> MGIVEEAHNVKVLGTGSRFIVLAHGFGTDQSVWKHLVPHLLEEFRVILYDNMGAGTTNPDYFDFERYSTLEGYAYDLLAILQELRVDSCIFVGHSVSAMIGTVASISRPDLFAKIIMISASPRYLNDSNYFGGFEQEDLDQLFNAMASNYKAWCSGFAPMAIGGDMESVAVQEFSRTLFNMRPDI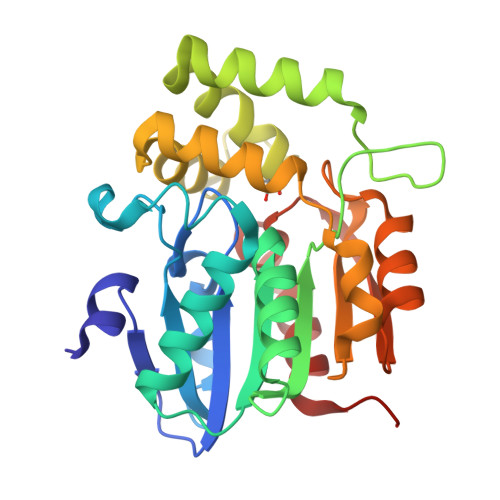ALSVLQTIFKSDMRQILCLVSVPCHIIQSMKDLAVPVVVAEYLHQHVGTESIVEVMSTEGHLPQLSSPDVVIPVILKHIRYDIVA> MDEFELIKRNTSEIISEEELREVLKKDEKSASIGFEPSGKIHLGHYLQIKKMIDLQNAGFDIIIALADLMAYLNQKGELDEIRKIGDYNKKVFEAMGLKAKYVYGSEFQLDKDYTLNVYRLALKTTLKRARRSMELIAREDENPKVAEVIYPIMQVNSIHYEGVDVAVGGMEQRKIH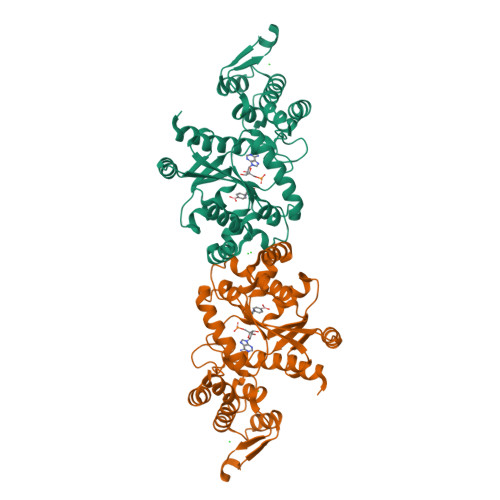MLARELLPKKVVCIHNPVLTGLDGEGKMSSSKGNFIAVDDSPEEIRAKIKKAYCPAGVVEGNPIMEIAKYFLEYPLTIKRPEKFGGDLTVNSYEELESLFKNKELHPMRLKNAVAEELIKILEPIRKRLSAHHHHHH> MSEFLTPERTVYDSGVQFLRPKSLDEFIGQENVKKKLSLALEAAKMRGEVLDHVLLAGPPGLGKTTLAHIIASELQTNIHVTSGPVLVKQGDMAAILTSLERGDVLFIDEIHRLNKAVEELLYSAIEDFQIDIMIGKGPSAKSIRIDIQPFTLVGSTTRSGLLSSPLRSRFGIILELDFYTVKE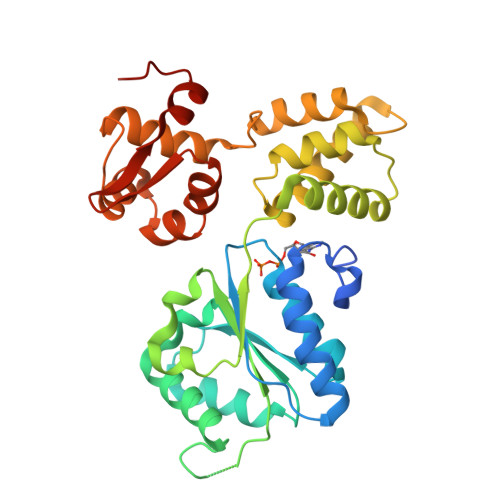LKEIIKRAASLMDVEIEDAAAEMIAKRSRGTPRIAIRLTKRVRDMLTVVKADRINTDIVLKTMEVLNIDDEGLDEFDRKILKTIIEIYRGGPVGLNALAASLGVEADTLSEVYEPYLLQAGFLARTPRGRIVTEKAYKHLKYEVPENRLF>SKWPEPVFGRLVSPGFPEKYGNHQDRSWTLTAPPGFRLRLYFTHFNLELSYRCEYDFVKLTSGTKVLATLCGQESTDTERAPGNDTFYSLGPSLKVTFHSDYSNEKPFTGFEAFYAAEDVDECRTSLGDSVPCDHYCHNYLGGYYCSCRVGYILHQNKHTCSALCSGQVFTGRSGFLSSPEYPQPYPKLSSCAYNIRLEEGFSI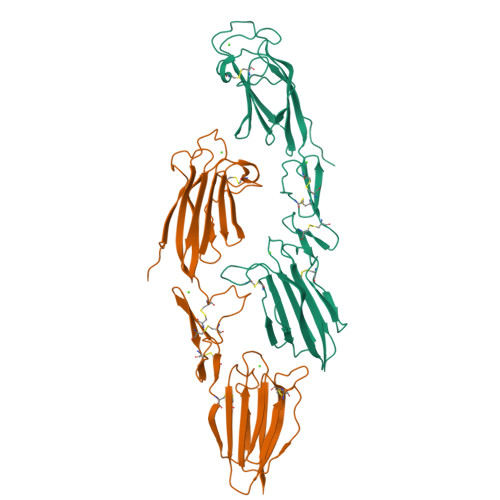TLDFVESFDVEMHPEAQCPYDSLKIQTDKREYGPFCGKTLPPRIETDSNKVTITFTTDESGNHTGWKIHYTSTA[2x]>[2x]AERPTLPIPDLLTTDARNRIQLTIGAGQSTFGGKTATTWGYNGNLLGPAVKLQRGKAVTVDIYNQLTEETTLHWHGLEVPGEVDGGPQGIIPPGGKRSVTLNVDQPAATCWFHPHQHGKTGRQVAMGLAGLVVIEDDEILKLMLPKQWGIDDVPVIVQDKKFSADGQIDYQLDVMTAAVGWFGDTLLTNGAIYPQHAAPRGWLRLRLLNG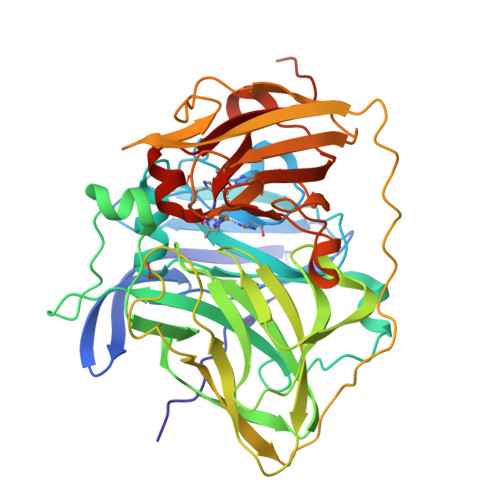CNARSLNFATSDNRPLYVIASDGGLLPEPVKVSELPVLMGERFEVLVEVNDNKPFDLVTLPVSQMGMAIAPFDKPHPVMRIQPIAISASGALPDTLSSLPALPSLEGLTVRKLQLSMDGGANKINGQAFDMNKPMFAAAKGQYERWVISGVGDMMLHPFHIHGTQFRILSENGKPPAAHRAGWKDTVKVEGNVSEVLVKFNHDAPKEHAYMAHCHLLEHEDTGMMLGFTVGHHHHH> GLRFPSKMFG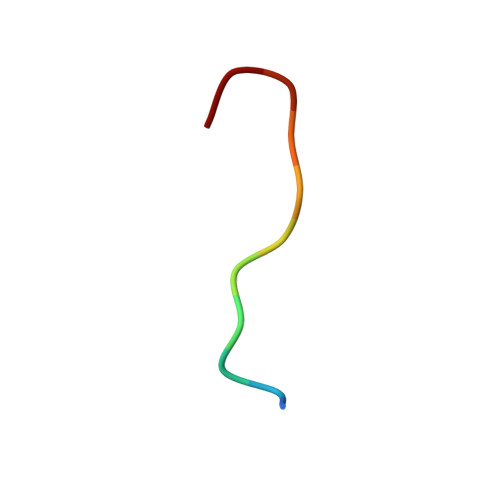G> VKDTYTDRLDDWNGIIAGNQYYDSKNDQMAKLNQELEGKVADSLSSISSQADRIYLWEKFSNYKTSANLTATYRKLEEMAKQVTNPSSRYYQDETVVRTVRDSMEWMHKHVYNSEKSIVGNAADYEIGTPRAINNTLSLMKEYFSDEEIKKYTDVIEKFVPDPEHFRKTTDNPVKALGGNLVDMGRVKVIAGLLRKDDQEISSTIRSIEQVFKLVDQGEGFYQDGSYIDHTNVAYTGAYGNVLIDGLSQLLPVIQKTKNPIDKDKMQTMYHWIDKSFAPLLVNGELMDMSRGRSISRANSEGHVAAVEVLRGIHRIADMSEGETKQRLQSLVKTIVQSDSYYDVFKN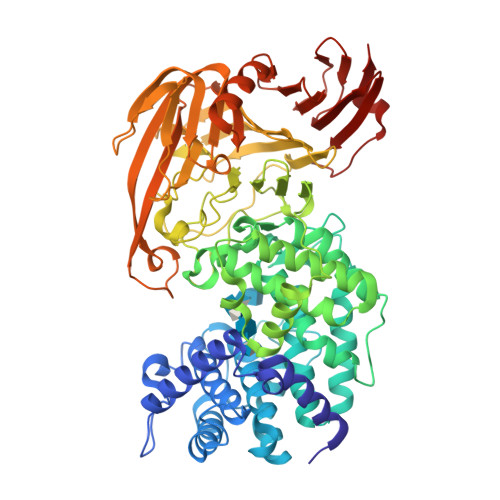LKTYKDISLMQSLLSDAGVASVPRTSYLSAFNKMDKTAMYNAEKGFGFGLSLFSSRTLNYEHMNKENKRGWYTSDGMFYLYNGDLSHYSDGYWPTVNPYKMPGTTETDAKRADSDTGKVLPSAFVGTSKLDDANATATMDFTNWNQTLTAHKSWFMLKDKIAFLGSNIQNTSTDTAATTIDQRKLESSNPYKVYVNDKEASLTEQEKDYPETQSVFLESSDSKKNIGYFFFKKSSISMSKALQKGAWKDINEGQSDKEVENEFLTISQAHKQNGDSYGYMLIPNVDRATFNQMIKELESSLIENNETLQSVYDAKQGVWGIVKYDDSVSTISNQFQVLKRGVYTIRKEGDEYKIAYYNPETQESAPDQEVFKKL>GSMSEDIRRGPGRPPKKRVVPNFERKGILEKPVRPQSRLEFSYDNPLIFKNLFIYFKNLKSKNILVRCTPTEITFFSRDQSQASFVIATIDGKNVNHYYASDVFWLGINRELVEKMFNSIDRSFLKITIVHRYDKPETLFFIFTDFDIDKECTYQITVSEPELDMDLIEMEKSISEERLKNYPLRWEFTSKQLKKTFSDLSNYTELVTIEKLGGDTPLHLYFQKFNSI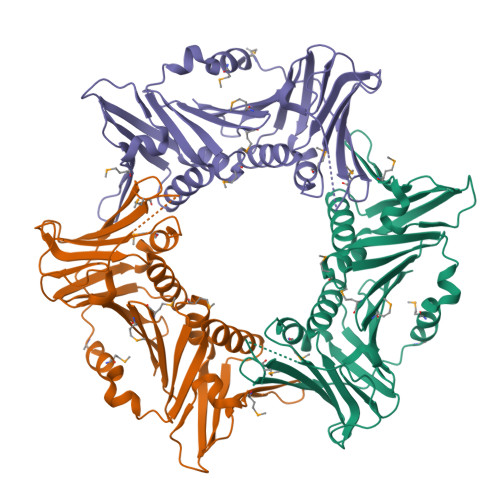SYHEMYKSSNKINLTSTIPKSQVFQINVKIAHIKSLASAMVTDKIRILCEENGNLIFQSEMDALMLNTITLNNTI[6x]> DDYYLN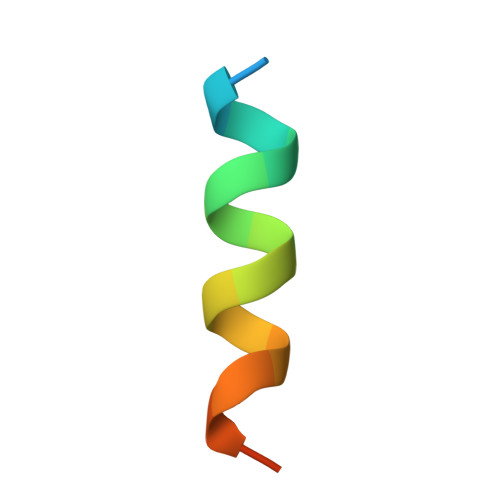LNQDEESLLRSRC> MYGFEAMTFNIHGGYLEAIVRGYRA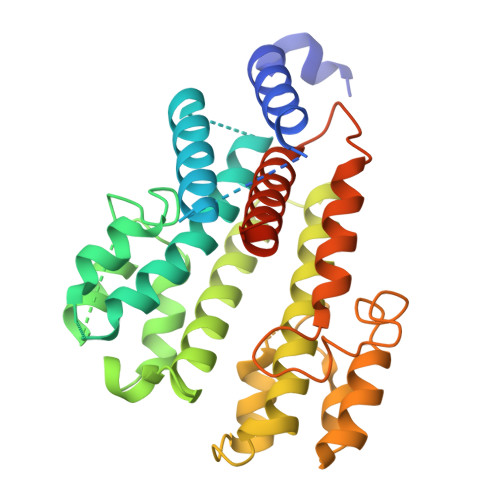GLLTAADYNNLCQCETLDDIKMHLSATEYGPYLQNEPSPLHTTTIVEKCTLKLVDEYKHMLCQATEPLSTFLEYITYGHMIDNVVLIVTGTLHERDVQELLEKCHPLGMFDSIATLAVAQNMRELYRLVLVDTPLAPYFSECITSEDLDDMNIEIMRNTLYKAYLEDFYKFCQKLGGATAEIMSDLLAFEADRRAVNITINSIGTELTRDDRRKLYSNFGLLYPYGHEELAVCEDIDQVRGVMEKYPPYQSIFSKLSYGESQMLDKAFYEEEVKRLCLAFEQQFHYGVFFAYMRLREQEIRNLMWISECVAQNQKSRVHDSVVFIF>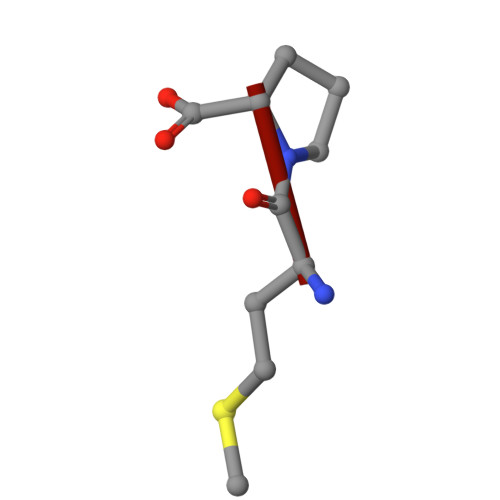 MP(4~{S})-5-[4-[[4-(2-ethyl-2-oxidanyl-butoxy)-3-methyl-phenyl]-methyl-phenyl-silyl]-2-methyl-phenoxy]-4-oxidanyl-pentanoic 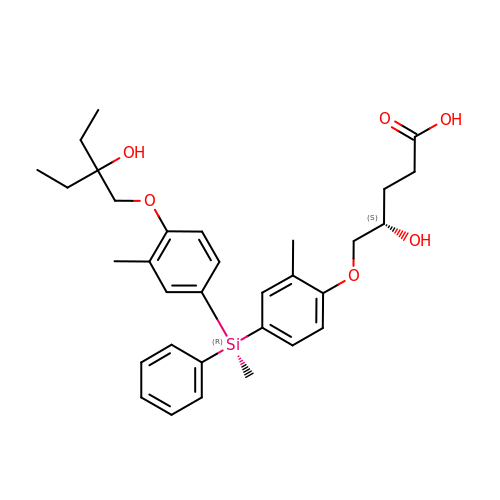acid | C32 H42 O6 Si | OGWGETOGIMXEHG-DGXSBJFJSA-N> AARATVAGGGRLMDRIRKWYYNAAGFNKYGLMRDDTLYEDDDVKEALKRLPKDLYNERMFRI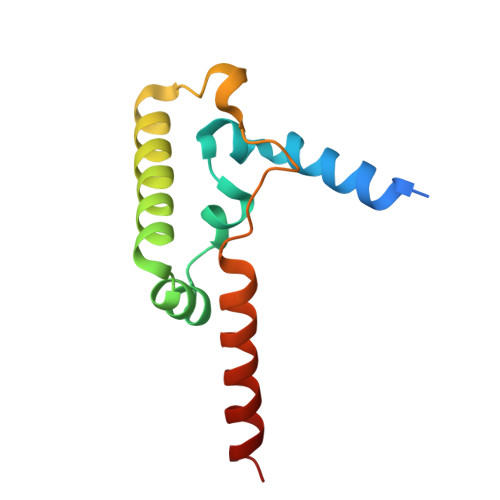KRALDLSLKHRILPKEQWVKYEEDKPYLEPYLKEVIRERLEREAWNKK[(1S,2S)-1,2-DIHYDROXYPROPYL]PHOSPHONIC ACID | C3 H9 O5 P | 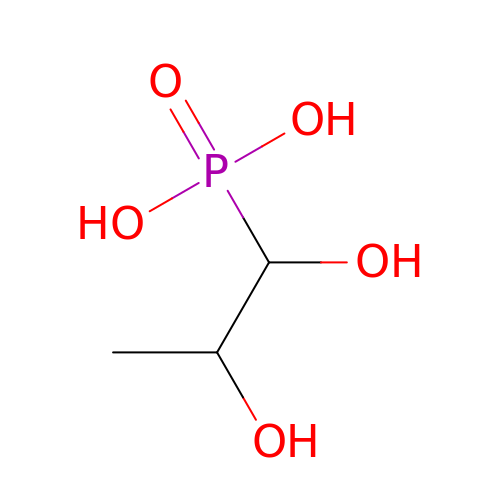MXMXXUIOCREOTJ-HRFVKAFMSA-N>[7x]AYTKISDVIVPELFNPYVINTTTQLSAFFQSGIAATDDELNALAKKAGGGSTLNMPYWNDLDGDSQVLNDTDDLVPQKINAGQDKAVLILRGNAWSSHDLAATLSGSDPMQAIGSRVAAYWAREMQKIVFAELAGVFSNDDMKDNKLDISGTADGIYSAETFVDASYKLGDHESLLTAIGMHS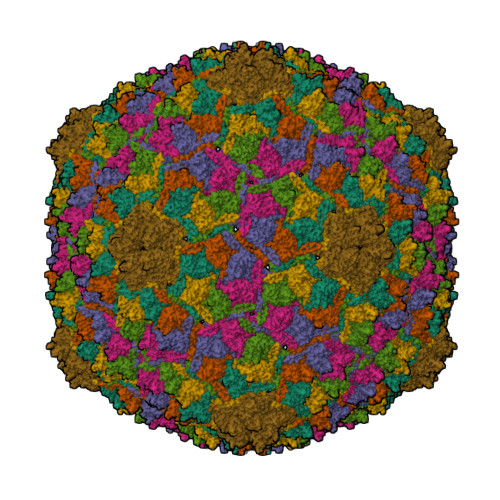ATMASAVKQDLIEFVKDSQSGIRFPTYMNKRVIVDDSMPVETLEDGTKVFTSYLFGAGALGYAEGQPEVPTETARNALGSQDILINRKHFVLHPRGVKFTENAMAGTTPTDEELANGANWQRVYDPKKIRIVQFKHRLQA>SPILGYWKIKGLVQPTRLLLEYLEEKYEEHLYERDEGDKWRNKKFELGLEFPNLPYYIDGDVKLTQSMAIIRYIADKHNMLGGCPKERAEISMLEGAVLDIRYGVSRIAYSKDF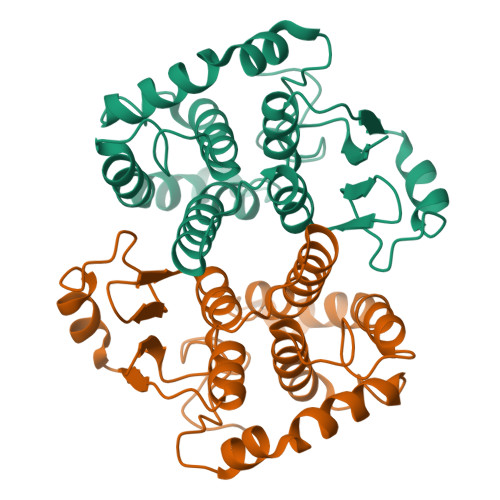ETLKVDFLSKLPEMLKMFEDRLCHKTYLNGDHVTHPDFMLYDALDVVLYMDPMCLDAFPKLVCFKKRIEAIPQIDKYLKSSKYIAWPLQGWQATFGGGDHPPKSDLVPR[2x]> MADSELVAQWEKVQIKTFTKWVNMHLAKKGRKINDVTTDFKNGVELCALLEIIGETTIKCVTNPKMRIQMTENLDKALRFIQSRDVKLTGIGPTDIVDGNVKLTLGLVWTLILRFAISELSAEGLSAKQGLLLWCQKKCEPYPVKVENFSESF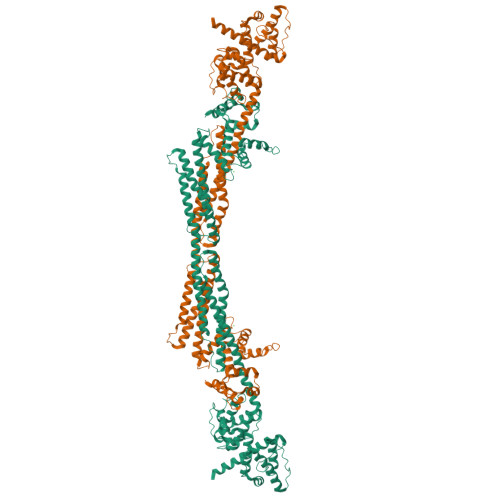KDGKVFCALIHRHRPDLLDWETVGEDDRANLEKAFDVAEKELGIPKLLDVDDIVNMPRPDERSVMTYVAALYKVFSSNDQVEKAGKRAGNFLDLLRATEGMVHDYEQRAQALKENIEAAINKMNGVEPSDEYHQVKEQINETKNYRKGDKRAFIKEQGDLATLFGQINSKLRGMKRPVYVAPEGLDPKSLEGYIANISEAERALRSKLNTAMRNCLIALRKAFADPANATDAKINEYRTFVTDETSEAPLEEQVATLKAKLEELKQVEAQLPPIEEAEKACGDANIEDNEYTDVSFDDLQFNYEQTVSMFEKKIVYIEAQINEASSGVTAEQMQEFKQSFDAFDGNHDGILDKLEFRSCLSSMGLIDIDFTGGEDAQYDAIYNNVTKGENGVSFDNYVQYMKEKNDENPSPEQLNEIFSTIAAGKDSITETDMQKAGMSAEQIEYVKANLPQKGDGYDYAAWVKTN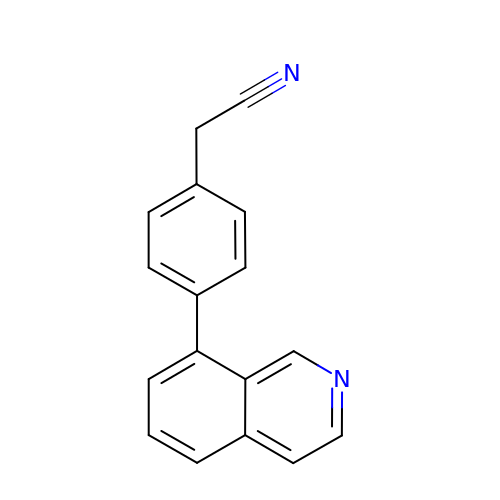[4-(isoquinolin-8-yl)phenyl]acetonitrile | C17 H12 N2 | VIKXCGPZKMDDCE-UHFFFAOYSA-N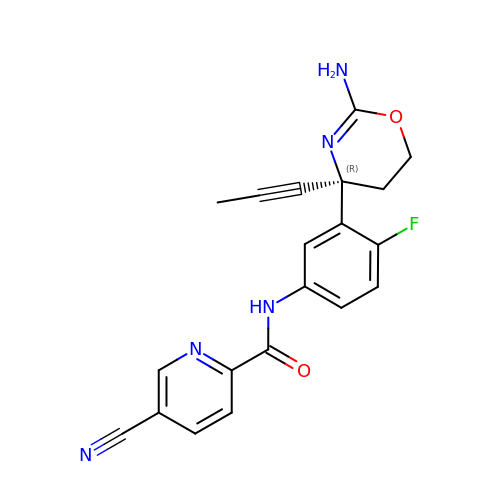N-[3-[(4R)-2-azanyl-4-prop-1-ynyl-5,6-dihydro-1,3-oxazin-4-yl]-4-fluoranyl-phenyl]-5-cyano-pyridine-2-carboxamide | C20 H16 F N5 O2 | DWCWSXLKLMTBSD-FQEVSTJZSA-N> MRGSHHHHHHGSEEASSTGRNFNVEKINGEWHTIILASDKREKIEDNGNFRLFLEQIHVLEKSLVLKFHTVRDEECSELSMVADKTEKAGEYSVTYDGFNTFTIPKTDYDNFLMAHLINEKDGETFQLMGLYGREPDLSSDIKERFAQLCEEHGILRENIIDLSNANRCLQARE

Recently, we observed a paradoxical enthalpy-driven thermodynamic binding signature in studies on a model ligand–protein interaction, namely the association of small hydrophobic ligands within the hydrophobic binding pocket of recombinant mouse major urinary protein (rMUP). In the case of rMUP we found that the binding pocket is suboptimally hydrated, a phenomenon that is increasingly being reported in other proteins. However, a negative change in heat capacity on binding (ΔCpb) is nonetheless observed in rMUP–ligand interactions, and is of similar or greater magnitude to that observed in typical ligand–protein interactions.[15–17] The serendipitous discovery that rMUP binds members of the primary aliphatic alcohol series as surrogate ligands permits a rigorous quantitative assessment of the solvation contribution to ΔCp, since the hydration thermodynamics of these ligands are very well characterized. We conclude that the characteristic negative change in heat capacity observed in rMUP–ligand complexation is largely determined by ligand desolvation, with minor contribution from desolvation of the protein.

We sought to determine whether this excess could be attributed to expulsion of residual ordered solvent water molecules from the protein binding pocket. We, therefore, solved the structure in the presence of an alternative cryoprotectant, paratone-N, which does not bind in the binding pocket of the protein. The structure revealed the presence of four ordered solvent water molecules in the apo structure. By assuming that a given water molecule in contact with each solute occupies an area of about 9 Å2, they concluded that the increase in heat capacity on solvation of hydrophobic groups amounts to about 13 J mol−1 K−1 per water molecule. These data suggest that the contribution to ΔCpb from loss of ordered water molecules from the protein-binding pocket is at most about −50 J mol−1 K−1, since the crystal structures of the rMUP–alcohol complexes also contain between one and three ordered water molecules. There exists the formal possibility that disordered water molecules within the binding pocket might also contribute to the thermodynamic binding signature. However, previous molecular dynamics simulations on uncomplexed rMUP suggested that on average only 3.5 water molecules are present in the binding pocket, which is in good agreement with the X-ray data. In the case of rMUP, the entropic contribution that would normally be expected to arise from protein desolvation is not present. Instead, the favourable enthalpic contribution that arises from solute–solute dispersion interactions, which also indirectly arises from solvation (or desolvation in this case), becomes the dominant term.Leniolisib | C21 H25 F3 N6 O2 | 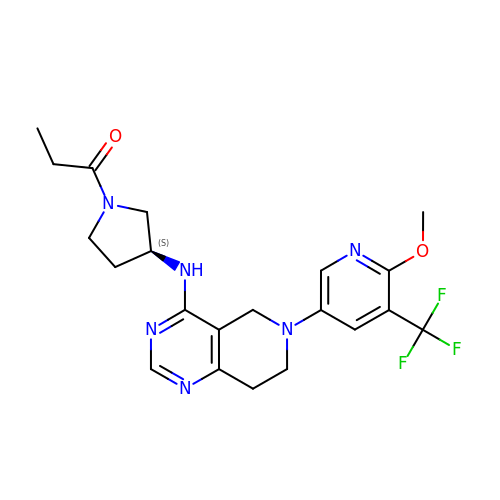MWKYMZXCGYXLPL-ZDUSSCGKSA-N>MILVTGGARSGKSRHAEALIGDAPQVLYIATSQILDDEMAARIQHHKDGRPAHWRTA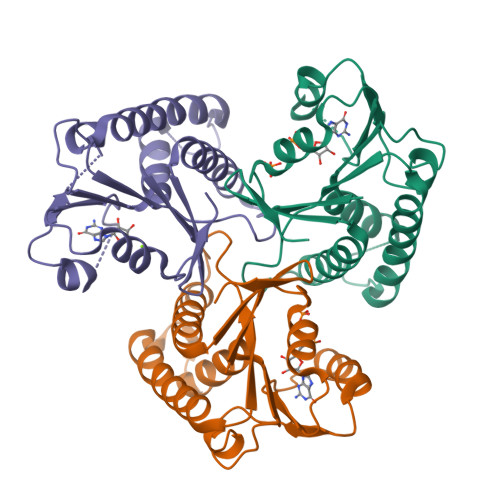ECWRHLDTLITADLAPDDAILLECITTMVTNLLFALGGENDPEQWDYAAMERAIDDEIQILIAACQRCPAKVVLVTNEVGMGIVPENRLARHFRDIAGRVNQRLAAAADEVWLVVSGIGVKIK[3x]> MAEEEEVEEGRSSSSAILDLPEPLLLHILSFLTDVRSRHRAALACGRMRAAERATRSELSLRGDPRSPGFLFLSHAFRFPALEHLDLSLVSPWGHPLLSSVPPCGGGGGGAPSASSSSGMNVYHPEAISEQNAFIAARLAGCFPAVTSLAVYCRDPTTLANLTPHW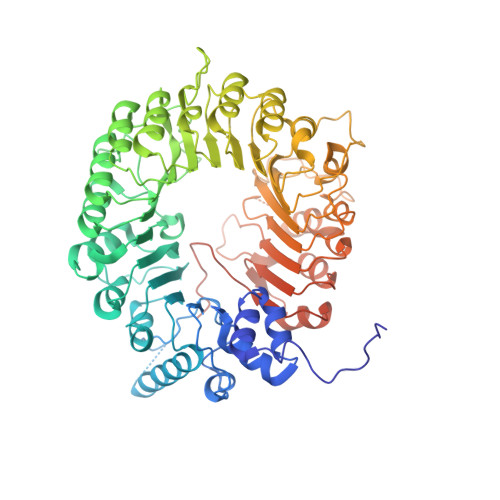QASLRRVKLVRWHQRPPTLPDGADLEPLLETCAALRELDLSEFYCWTEDVVRALTTHPSATAALTHLDLGLAAATDGFKSSELGPIAASCPNLRKLVAPCLFNPRFSDCVGDDALLSLATSCPRLTVLRLSEPFEAAANIQREEAAITVAGLVAFFAALPALEDFTMDLQHNVLEAAPAMEALARRCPRIKFLTLGSFQGLCKASWLHLDGVAVCGGLESLYMKNCQDLTDASLAAIGRGCRRLAKFGIHGCDLVTSAGIRRLAFTLRPTLKEVTVLHCRLLHTAECLTALSPIRDRIESLEINCVWNTTENLYFQSLGSWEMLRSLSLWFSAGQLLSPLISAGLDSCPVLEEISIKVEGDCRTCPRPAPRTIFGLSDLAGFPVLAKMKLDLSEAVGYALTAPTGQMDLSLWERFYLHGIESLQTLYELDYWPPQDKDVHHRSLTLPAVGLIQRCVGLRKLFIHGTTHEHFMTFFLSIPNLRDMQLREDYYPAPENDLMFTEMRAESWLRFEVQLNSRQIDK> GMENQEVVLSIDAIQEPEQIKFNMSLKNQSERAIEFQFSTGQKFELVVYDSEHKERYRYSKEKMFTQAFQNLTLESGETYDFSDVWKEVPEPGTYEVKVTFKGRAENLKQVQAVQQFEVK

The structure of IPI is a variant of the all-beta, immunoglobulin (Ig) fold. It is possible that IPI is important for protein-protein interactions, of which inhibition of Isp1 is one. IPI homologues are found in both bacteria and archaea, but no homologues have been detected in eukaryotes.

Bacillus subtilis was determined to 2.6 Å resolution by the MAD method. 29 shows that 98.0% of the residues are in favoured regions, with no outliers. Two residues, Lys 86 and Glu 87, are flagged as having unusual Ramachandran plot properties by the PDB validation report although not with Molprobity. Electron density for them strongly supports their modelled conformations. The structure has an unusual Ig-like fold. Protruding loops on the right hand side form a wedge shape. Remarkably, we find that the region at the edge of the IPI wedge structure could interact with subtilisin in a manner strongly reminiscent of inhibition modes of other subtilisin family inhibitors. Chagasin and amoebiasin have similar topologies, but the order of the beta strands differs significantly between these two I42 family members and IPI. This implies that IPI is not closely related to the I42 family, and that the similar folds may have been acquired independently by convergent evolution. However, the tertiary structure and docking predictions illustrate how it could feasibly inhibit its cognate enzyme.>[2x]SNAIRPTIGQQMETGDQRFGDLVFRQLAPNVWQHTSYL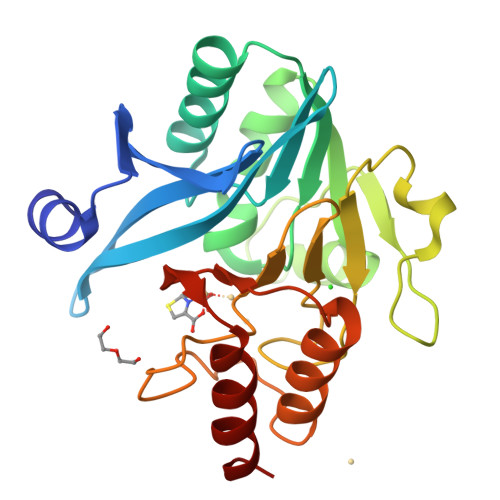DMPGFGAVASNGLIVRDGGRVLVVDTAWTDDQTAQILNWIKQEINLPVALAVVTHAHQDKMGGMDALHAAGIATYANALSNQLAPQEGMVAAQHSLTFAANGWVEPATAPNFGPLKVFYPGPGHTSDNITVGIDGTDIAFGGCLIKDSKAKSLGNLGDADTEHYAASARAFGAAFPKASMIVMSHSAPDSRAAITHTARMADKLR>[5x]SKARVEALANSRHVLDFQTAFDRPYQFMALSEQATIEWGNTGDANPHAEGGFVKRHGDDSAFGAYFGRRSADFSEAVQTVRDASSHHHHHHGSSNPAFADLMFEQNGLNLFYASKMGEWTWGVTAKYSNGKNED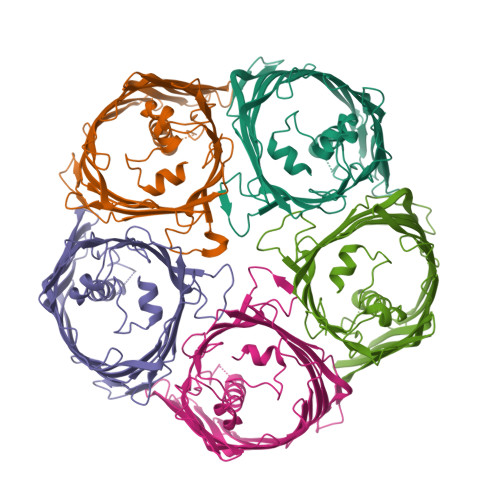PTVGTKATSAGVAVAASNGTWDFELVQGFTGKSELDNGTVTAEVESKGLTNVTVGYHMSPEMEVYGNVKMSKVEADLNGTPIEVETTSYKVGMVNTLAKSEEGNFFYGVEVASTKVKDDSESLLLPVYMGVEHNAASWLVLRASVAQNVILNETKDDATGNKTDEDSTRMAAGAGIKFGKSVIDASFAGSTTGVINANNLFSQVAYTYTF>DFAEYFESLGGQVIETGYLVTLEKGKIRKAEKGEKIIGVISET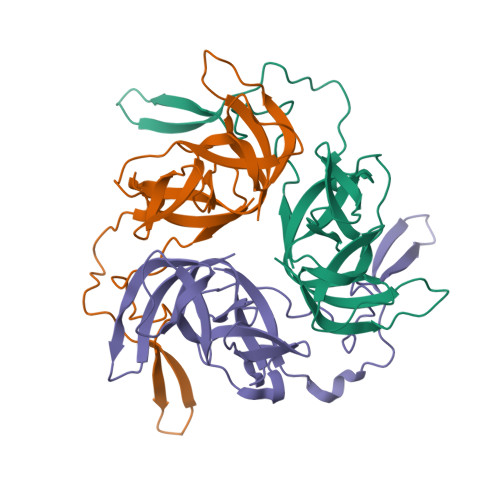AGFVLGESSFEWQGAVLKNEFGGIIYEEVTTEDGVKFKRPLPNPDFDPNKNYIPRSQRREWHVVGLLGQIAVRIDETVKQGHSIDAVGGVATDGDNFIVQEITTPYTKEKGYGVAIVLVK[3x]> VNYAAGLSPYADKGKCGLPEIFDPPEELERKVWELARLVWQSSSVVFHTGAGISTASGIPDFRGPHGVWTMEERGLAPKFDTTFESARPTQTHMALVQLERVGLLRFLVSQNVDG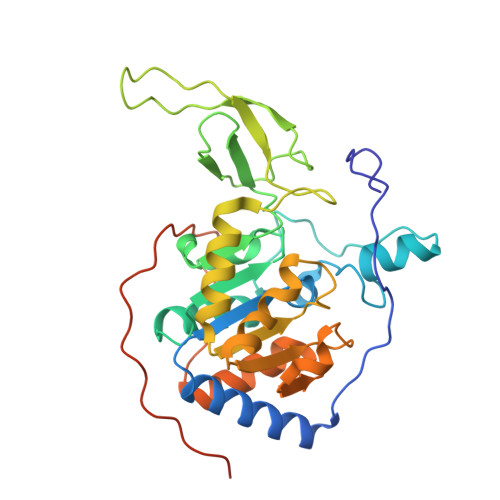LHVRSGFPRDKLAELHGNMFVEECAKCKTQYVRDTVVGTMGLKATGRLCTVAKARGLRACRGELRDTILDWEDSLPDRDLALADEASRNADLSITLGTSLQIRPSGNLPLATKRRGGRLVIVNLQPTKHDRHADLRIHGYVDEVMTRLMKHLGLEIPAWDGPRVLERALPPLPRPPTPKLEPKEESPTRINGSIPAGPKQE Human ATP:cob(I)alamin adenosyltransferase (ATR) is a mitochondrial enzyme that catalyzes an adenosyl transfer to cob(I)alamin, synthesizing 5′-deoxyadenosylcobalamin (AdoCbl) or coenzyme B12. ATR is also a chaperone that escorts AdoCbl, transferring it to methylmalonyl-CoA mutase, which is important in propionate metabolism. Mutations in ATR lead to methylmalonic aciduria type B, an inborn error of B12 metabolism. Human ATR is a homotrimer with active sites that are located at the subunit interfaces.

The structure of R190C ATR·ATP represents the highest resolution structure reported so far for human ATR. An alignment of these two structures showed that the R190C mutation did not elicit a major structural change in the protein (Cα RMSD = 0.5). All six monomers in the asymmetric unit were identical and ATP could be modeled with an occupancy of one per monomer. In this structure, a complete ordering of loops, except for the first 50 residues, was observed. ATP induced ordering of residues 68 to 80 into a β-hairpin, forming the roof of the active site. An overlay of the ATP binding sites shows that many of the interactions that stabilize ATP binding are retained in the R190C ATR. Although the overall mode of ATP binding is unperturbed, the R190C mutation leads to the loss of multidentate electrostatic interactions between Arg-190 and ATP, possibly contributing to the higher KM(ATP) value and in turn, the higher KD values for cob(II)alamin (in the presence of ATP) and AdoCbl (±PPPi). Interestingly, the salt bridge between Arg-190 and the ribose oxygen is replaced by a hydrogen bond between Cys-190 and the ribose oxygen mediated via a bridging water. The salt bridges between Arg-190 and the α-phosphate oxygens are however, lost. The position of the C5′ carbon, which is attacked by cob(I)alamin, is unchanged in the crystal structure of the R190C mutant.

>[6x]MPKIYTKTGDKGFSSTFTGERRPKDDQVFEAVGTTDELSSAIGFALELVTEKGHTFAEELQKIQCTLQDVGSALATPCSSAREAHLKYTTFKAGPILELEQWIDKYTSQLPPLTAFILPSGGKISSALHFCRAVCCRAERRVVPLVQMGETDANVAKFLNRLSDYLFTLARYAAMKEGNQEKIYMKNDPSAESEGL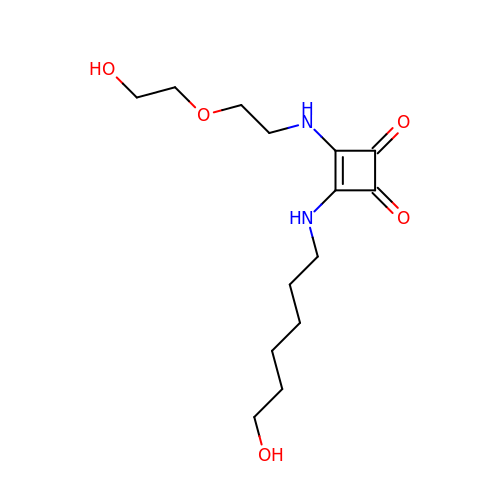3-{[2-(2-hydroxyethoxy)ethyl]amino}-4-[(6-hydroxyhexyl)amino]cyclobut-3-ene-1,2-dione | C14 H24 N2 O5 | RJWRZWAPNJTDAQ-UHFFFAOYSA-N>[8x]MNGKIALE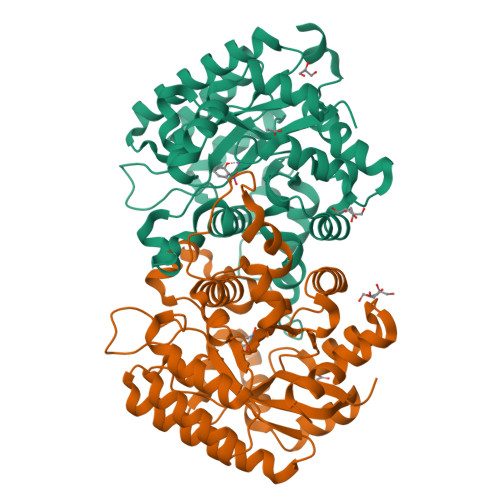EHFATEETLMDSAGFVPDKDWPELRSRLLDIQDRRVRLMDEHGIETMILSLNAPAVQAIADSTRANETARRANDFLAEQVAKQPTRFRGFAALPMQDPELAARELERCVKELGFVGALVNGFSQDNRSAVPLYYDMAQYWPFWETVQALDVPFYLHPRNPLPSDARIYDGHAWLLGPTWAFGQETAVHALRLMGSGLFDKYPALKIILGHMGEGLPYSMWRIDHRNAWIKTTPKYPAKRKIVDYFNENFYLTTSGNFRTQTLIDAILEIGADRILFSTDWPFENIDHAADWFENTSISEADRKKIGWGNAQNLFKLNRAENLYFQSHHHHHHWSHPQFEK Norflurazon | 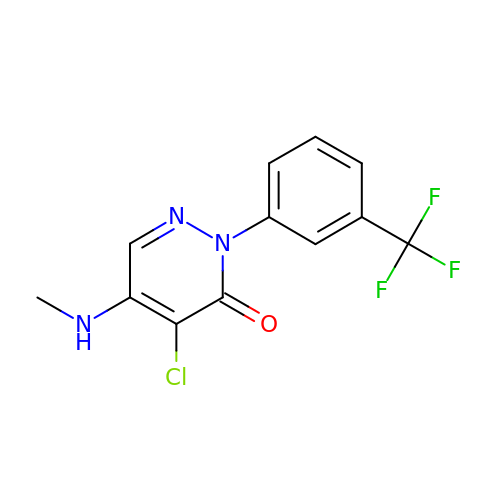C12 H9 Cl F3 N3 O | NVGOPFQZYCNLDU-UHFFFAOYSA-N>AKTYTLTDYLKNTYRLKLYSLRWISDHEYLYKQENNILVFNAEYGNSSVFLENSTFDEFGHSINDYSISPDGQFILLEYNYVKQWRHSYTASYDIYDLNKRQLITEERIPNNTQWVTWSPVGHKLAYVWNNDIYVKIEPNLPSYRITWTGKEDIIYNGITDWVYEEEVFSAYSALWWSPNGTFLAYAQFNDTEVPLIEYSFYSDESLQYPKTVRVPYPKAGAVNPTVKFFVVNTDSLSSVTNATSIQITAPASMLIGDHYLCDVTWATQERISLQWLRRIQNYSVMDICDYDESSGRWNCLVARQHIEMSTTGWVGRFRPSEPHFTLDGNSFYKIISNEEGYRHICYFQIDKKDCTFITKGTWEVIGIEALTSDYLYYISNEYKGMPGGRNLYKIQLSDYTKVTCLSCELNPERCQYYSVSFSKEAKYYQLRCSGPGLPLYTLHSSVNDKGLRVLEDNSALDKMLQNVQMPSKKLDFIILNETKFWYQMILPPHFDKSKKYPLLLDVYAGPCSQKADTVFRLNWATYLASTENIIVASFDGRGSGYQGDKIMHAINRRLGTFEVEDQIEAARQFSKMGFVDNKRIAIWGWSYGGYVTSMVLGSGSGVFKCGIAVAPVSRWEYYDSVYTERYMGLPTPEDNLDHYRNSTVMSRAENFKQVEYLLIHGTADDNVHFQQSAQISKALVDVGVDFQAMW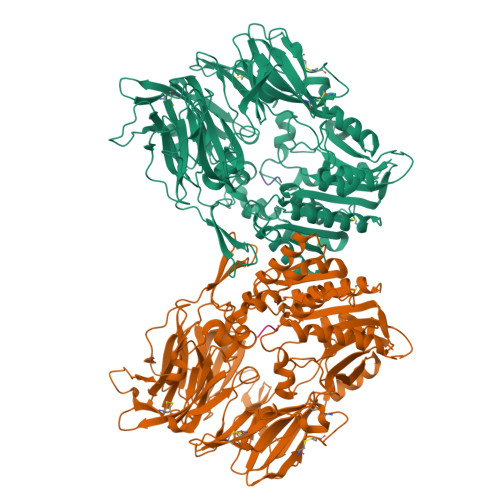YTDEDHGIASSTAHQHIYTHMSHFIKQCFSL[2x];>VAMP[2x]>MAHHHHHHGMTRTRSGSLAAGGLNWASLPLKLFAGGNAKFWHPADIDFTRDRADWEKLSDDERDYATRLCTQFIAGEEAVTEDIQPFMSAMRAEGRLADEMYLTQFAFEEAKHTQVFRMWLDAVGISEDLHRYLDDLPAYRQIFYAELPECLNALSADPSPAAQVRASVTYNHIVEGMLALTGYYAWHKICVERAILPGM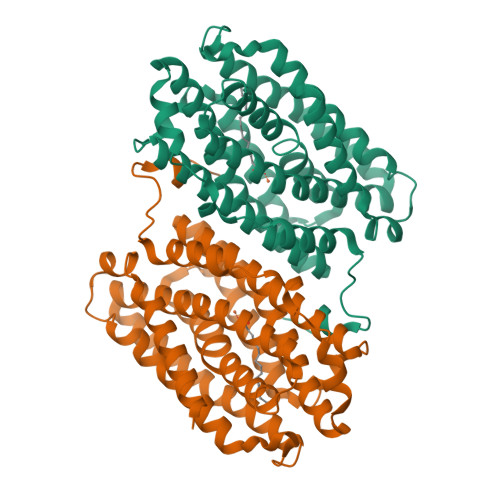QELVRRIGDDERRHMAWGTFTCRRHVAADDANWTVFETRMNELIPLALRLIEEGFALYGDQPPFDLSKDDFLQYSTDKGMRRFGTISNARGRPVAEIDVDYSPAQLEDTFADEDRRTLAAASA[4x]[[(2~{R},3~{R},4~{S},5~{R})-4-fluoranyl-5-(5-iodanyl-4-methyl-pyrrolo[2,3-d]pyrimidin-7-yl)-3-oxidanyl-oxolan-2-yl]methoxy-oxidanyl-phosphoryl] 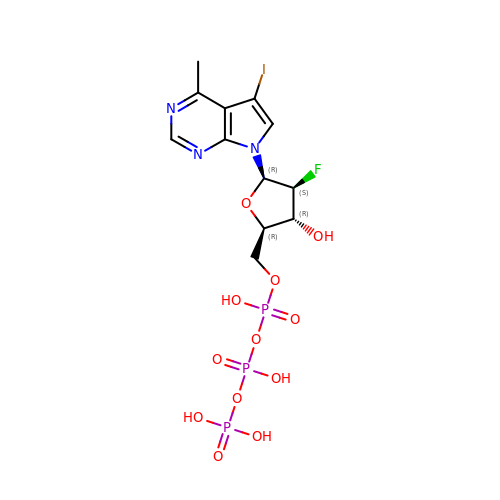phosphono hydrogen phosphate | C12 H16 F I N3 O12 P3 | SDPCZQPAUGWGIT-DLYFRVTGSA-N>[6x]MKIGIVTGIPGVGKSTVLAKVKEILDNQGINNKIINYGDFMLATALKLGYAKDRDEMRKLSVEKQKKLQIDAAKGIAEE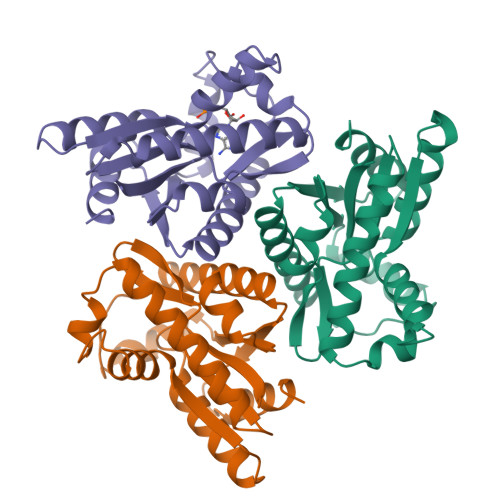ARAGGEGYLFIDTHAVIRTPSGYLPGLPSYVITEINPSVIFLLEADPKIILSRQKRDTTRNRNDYSDESVILETINFARYAATASAVLAGSTVKVIVNVEGDPSIAANEIIRSMK2-amino-7-{[(3R,4R)-3-hydroxy-4-(hydroxymethyl)pyrrolidin-1-yl]methyl}-3,5-dihydro-4H-pyrrolo[3,2-d]pyrimidin-4-one | C12 H17 N5 O3 | 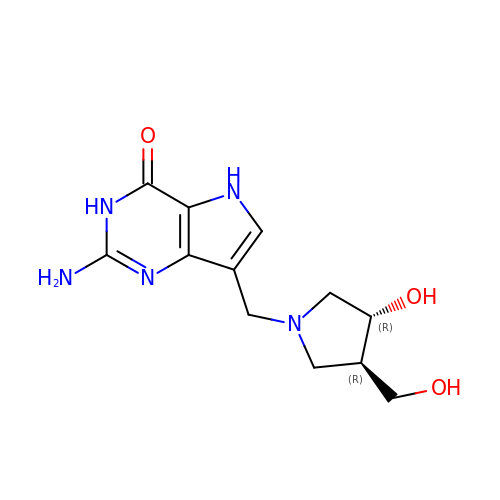GSPTUGDLYPMLCQ-SFYZADRCSA-N>MSSFHLDDINWQPNIEGVYNSEQRFNLNDYFTSEKVPGDGNCFFYSVSFLLFESLSEWRSIKNTIASFAAANWGQCVQAKLNYANSSDYRADMLRNYYWGGSVEAEILSKALNITIILWEADVSENVVTATKYGPGLVSTALNLKLCQGHIEPLQLMKLVDQDVLRKSGSHHHHHH[2x]

One specific mechanism used by nairoviruses is the production of a deubiquitinating enzyme, termed the vOTU, that disrupts the innate immune response. Interestingly, the nairoviral L segment also encodes a viral homologue of the ovarian tumor protease (OTU) at the N-terminus. Instead, the vOTU’s primary function appears to be the reversal of post-translational modifications by ubiquitin (Ub) and the Ub-like protein interferon stimulated gene product 15 (ISG15). Each vOTU possesses a seven-stranded beta sheet as the core feature, with five major alpha helices framing the rest of the structure.

The vOTUs from DGKV, QYBV, and TAGV readily crystallized and were solved to 1.62 Å, 1.65 Å, and 2.05 Å, respectively. DGKV vOTU, consistent with its low Ub-AMC activity, possesses very low activity for the di-Ub FRET substrates, regardless of the linkage. In DGKV vOTU, aspartate is replaced by a glutamate that alters the spatial dynamics of the catalytic triad, possibly contributing to a less rigid structure that allows the histidine to adopt the alternate conformation. While atypical for the vOTUs, it does not appear to be the cause of DGKV’s low DUB activity, as mutating the glutamate to an aspartate only further diminished activity. In DGKV vOTU, Trp73 packs with the methylene group of Ser86 on one side and the aliphatic portion of Lys80’s side chain on the other. Lys80 itself is stabilized in this permissive conformation by hydrogen bond pairing with the carbonyl of Gly74. In DGKV vOTU, Gln78 within the selectivity helix is central to the interaction, pairing with both Ser102 and Tyr133 by hydrogen bonding. In contrast, the DGKV and QYBV vOTUs possess more polar residues, including asparagine, glutamate, and threonine for DGKV and glutamine and lysine in QYBV. Interestingly, changing the pocket in DGKV vOTU failed to improve activity. This suggests that some vOTUs lacking any outright DUB activity may have evolved to a degree that prevents the generation of this activity through simple changes to better accommodate Leu8 in Ub.2-(5-{[(2S)-2-amino-3-phenylpropyl]oxy}pyridin-3-yl)-8,9-dimethoxybenzo[c][2,7]naphthyridin-4-amine | C28 H27 N5 O3 | 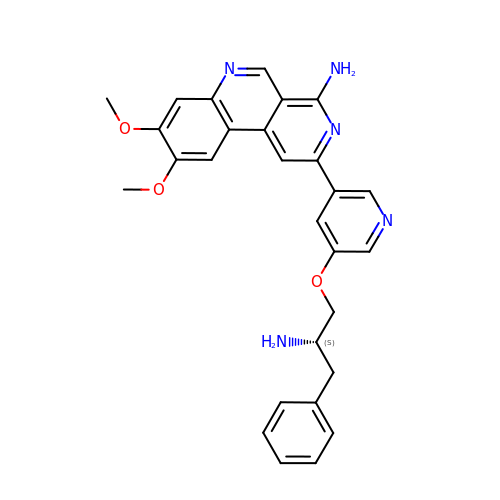XNXUJUXYVTYIGP-IBGZPJMESA-N>[12x]MATHKPINILEAFAAAPPPLDYVLPNMVAGTVGALVSPGGAGKSMLALQLAAQIAGGPDLLEVGELPTGPVIYLPAEDPPTAIHHRLHALGAHLSAEERQAVADGLLIQPLIGSLPN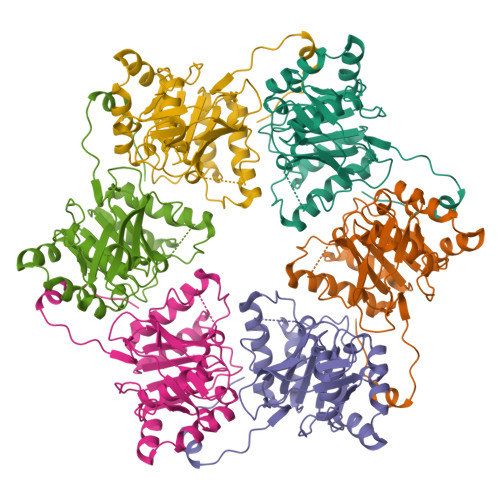IMAPEWFDGLKRAAEGRRLMVLDTLRRFHIEEENASGPMAQVIGRMEAIAADTGCSIVFLHHASKGAAMMGAGDQQQASRGSSVLVDNIRWQSYLSSMTSAEAEEWGVDDDQRRFFVRFGVSKANYGAPFADRWFRRHDGGVLKPAVLERQRKSKGVPRGEA Glutathione synthetase catalyses the synthesis of the low molecular mass thiol glutathione from l-γ-glutamyl-l-cysteine and glycine. The enzyme belongs to the ATP-grasp family, a group of enzymes known to undergo conformational changes upon ligand binding. First glutamylcysteine synthetase is responsible for the ligation of cysteine to glutamate and then glutathione synthetase (GS) converts the dipeptide to GSH by addition of glycine. The TbGS subunit is composed of two domains, a large “core” domain and a smaller “lid” domain that together form an ATP-grasp fold.

We have determined a low-resolution crystal structure of the parasite enzyme TbGS in complex with the product GSH. Four molecules are present in the asymmetric unit, forming two dimers consisting of subunits A with B, and C with D. The subunits are very similar in structure with r.m.s.d. values of 0.9 Å (A–B), 0.9 Å (A–C) and 0.8 Å (A–D) when they are superimposed with SSM. Size exclusion chromatography indicated that TbGS is a dimer in solution, and the asymmetric unit was found to comprise two such dimers, subunits A–B and C–D. The TbGS dimer is formed in a similar manner to that observed for the ScGS and HsGS with a non-crystallographic twofold rotation axis relating the subunits to each other. The lid domain is poorly resolved in the electron density map, with only a short section of anti-parallel β-sheet observed in subunits B, C and D. Subunit A displayed greater order in this region, allowing for model building of all but a short sequence between residues 443 and 446. In TbGS, the lid domain in subunit A is considered to be in an open position. Despite attempts to co-crystallize TbGS with ATP or the non-hydrolysable AMP-PNP, these ligands were not observed. The GSH binding site is positioned over the top of a loop linking β6 to α7, with further interactions to residues from the loops that link β8 to α10 and β13 to α12. The γ-glutamyl moiety forms salt bridge interactions with Arg324 and hydrogen bonds to Ser150, Glu264 and Asn266. The cysteine carbonyl and amide groups potentially form hydrogen bonds to Arg119 and Ser148 respectively. The glycinyl carboxylate is placed to form salt bridge interactions with TbGS Arg530 and again the interaction appears to be strictly conserved in HsGS with Arg450 and in ScGS with Arg467.

>[4x]NLYFQGHMVLKLLLELGAERYAEQFAAKCHELGMVMKESAGPGRVPVPVTLQPSMISRGEFGTLCCMQPLWNEAVDNTARNFTFLRDALQETAASDVNFTGKLLNMLQEVYLSGGPFQQLMLGIFRTDYMREGVYDKMLSTTASRWKNVEINTISCSFAGLSPLITEFHQHIAAYLQVLQKARGKEDDDGVENMSWIWGKGNCRLERSVSGDVVPKAIADAVRAWVEQQKFASLRASWEQFQQNEVGSGEIHQLGVLDTAPVVLVVVQENERNTADQYALLMRVLEEHRIRFIFRTLQELHLSLKLHSISPEQPPLAVVDGHYPIAVAYFRSTYVPEDFPTDATWAARLSLERSSAIKCPSIPYHLLTFKKLQQLLCDVDRVLVPVAFCGDSDKAGLLQRHFVPQYSLNPKEVGEEAVEKVIHDVLQRPDQFVLKPQLEGGGNLLSGETMVKALKATKEGDPVTYSKVRCEYVVMSRIQFHVSTGSLLARGDVVQLERNMCSEVGIFGVILSAAKGSSVGTNGSSVLFNTFAGYTVRSKPADADDGGVMAGVAALDSLAVVP> MIKQRTLKRIVQATGVGLHTGKKVTLTLRPAPANTGVIYRRTDLNPPVDFPADAKSVRDTMLCTCLVNEHDVRISTVEHLNAALAGLGIDNIVIEVNAPEIPIMDGSAAPFVYLLLDAGIDELNCAKKFVRIKETVRVEDGDKWAEFKPYNGFSLDFTIDFNHPAIDSSNQRYAMNFSADAFMRQ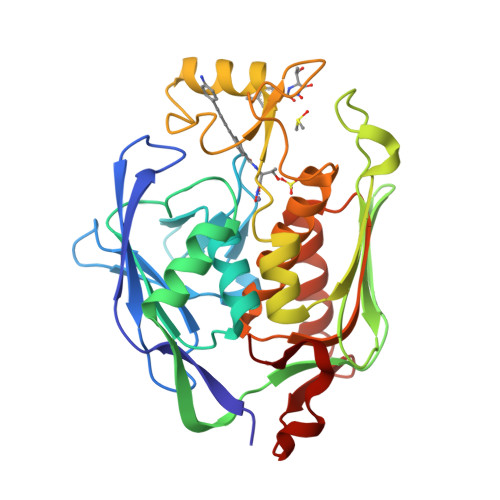ISRARTFGFMRDIEYLQSRGLCLGGSFDCAIVVDDYRVLNEDGLRFEDEFVRHKMLDAIGDLFMCGHNIIGAFTAYKSGHALNNKLLQAVLAKQEAWEYVTFQDDAELPLAFKAP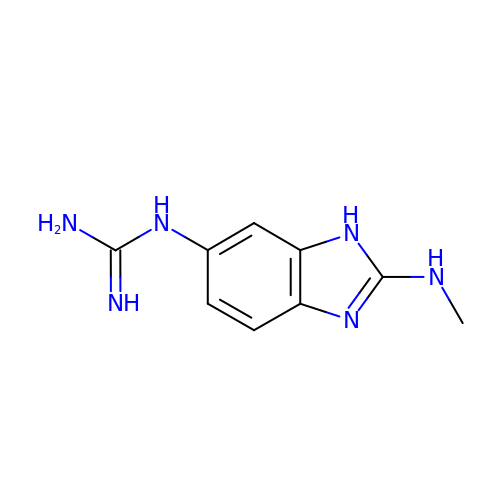N-[2-(methylamino)-1H-benzimidazol-6-yl]guanidine | C9 H12 N6 | VXGAAYFONQATFF-UHFFFAOYSA-N> HHHHHHHHPPSGADPMYAMPGNSGDLQCDDGKKRHIPPLSLLLSGYGSSEGRELDTSYTPKQWLWFLYVTSWARPFFTYASSGGASEATEGSSDNRSGSAYWGRLSFDELLKLSGSPIPPAMVSLWMGLCMPTDDVVQELRIMTEGKAEGRQRIYPFLPRVAESTFGRALRSLAVRQHISSWMPSHAGDVCAALDVLVRDTLEVIQNSADVRKTARVRCEERDASGEEALEGAFRSMLSASTTAPKVVEATTYRPLFDVKASIPEGGTAQVLIRVANAARLFAALSVEAFGRVKSECAVLLLAHINQRDAPEHVDARAYGVVTGVVEYAMAYRYCRDDGTGRCPLTCAALLLHRLVELQGIVEKDTAAGDRCMGMAVSASRFANMTVACIQELLFCVVAGDTVRWHREHQPDGVSVCPTAARTLTLHETDCLLQVFIPALLQQVGFEWPWSESLRHAKMLDRARTQHIVMEDGVRLDSRSVFEELLVSVARRTYGLRLRAILPQSFDVIAENIFVSIHDVPNEGKSSGGNPEKVADNSSSRFALPLYYRTAGEVLLEYFDRCGPSGITAEETERVLRRATDVQPMVVQLQALGGDTNGGITDCVSYCGELSRTVYFSAREKERLLQRYRCEVLLASLVVYTQLRTVSVVQQLTRQLAPLFEQLLLPLAHERTLSRCPV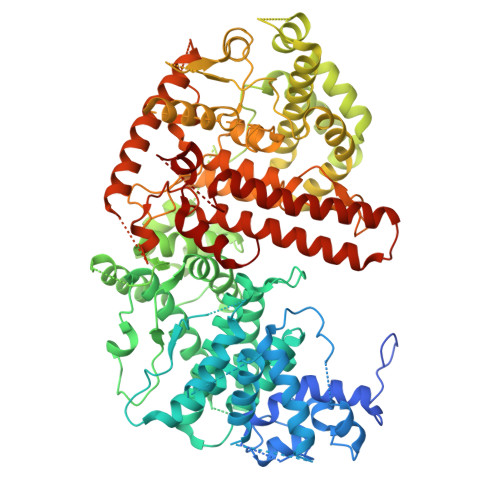IASRKGDGVDDNGTPLVDLTPEFKMLVDEIHYEFYPLEWVPEAVDAHIRQECGVREKEGAPYHEGGNGPPCFAQYSLFAAIAHQFGLVLEGNPRGFRGGDGSSSEVRTKAYRFFTLMLLNNLGDAVSSSCELDGAAALAATRRVKDCQDGSENCKQRQAAVRQRGGASFHSVVSACDVVVTMTQCLLPAHLSSHPRMATTGSMSNEWMRRVGEWTRSAYSKYTAYQQQVHGLDLPVPLISLYNSLTFDSVPLARETIRAVRSRLLEKMSVVTASPPGDVETAGKQLLEQHLSSLTVTLTAVGLLPLCVRGGSHVPCATQLLWASPFFSHELLHCGRYEVSV>MSKVVELLKQIQADASVFYVKVHNFHWNVKGMDFHPTHKATQEIYEQFADVFDDVAERVLQLGEMPYVTLADMLKAAKIKEESKTSFCSKEIAQAVLADYEYFLK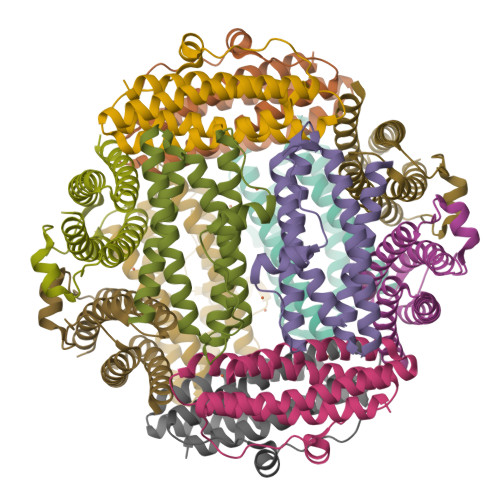LFTELSAQADSQGDKVSAAYADDKVGELQKAIWMLKSQLA[12x]>[5x]GQDMVSPPPPIADEPLTVNTGIYLIECYSLDDKAETFKVNAFLS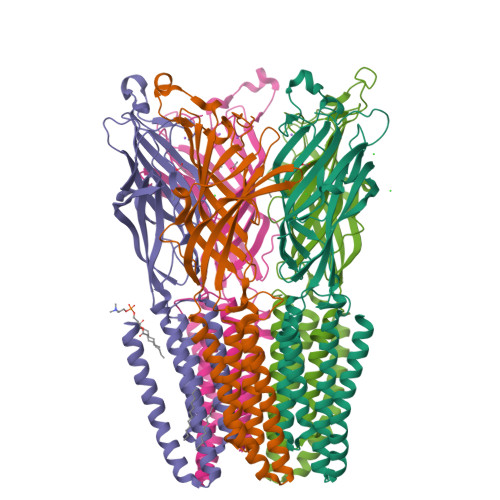LSWKDRRLAFDPVRSGVRVKTYAPEAIWIPEIRFVNVENARDADVVDISVSPDGTVQYLERFSARVLSPLDFRRYPFDSQTLHIYLIVRSVDTRNIVLAVDLEKVGKNDDVFLTGWDIESFTAVVKPANFALEDRLESKLDYQLRISRQYFSYIPNIILPMLFILFISWTAFWSTSYEANVTLVVSTLIAHIAFNILVETNLPKTPYMTYTGAIIFMIYLFYFVAVIEVTVQHYLKVESQPARAASITRASRIAFPVVFLLANIILAFLFFGF1-(4-{2-[(6-{4-[2-(dimethylamino)ethoxy]phenyl}furo[2,3-d]pyrimidin-4-yl)amino]ethyl}phenyl)-3-phenylurea 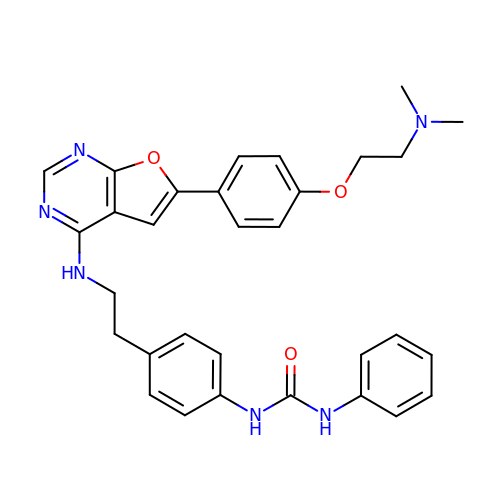| C31 H32 N6 O3 | GJFJLQXYFZSVOD-UHFFFAOYSA-N The N6-threonylcarbamoyladenosine (t6A) modification at position 37 of ANN-decoding tRNAs is one of the few modifications that are found in the three domains of life. In the first half of the reaction, YrdC utilizes ATP, L-threonine and bicarbonate to synthesize an unstable intermediate TCA, whose threonylcarbamoyl-moiety is subsequently transferred onto the adenosine at position 37 of the substrate tRNAs by the cooperative action of three proteins YeaZ, YgjD and YjeE. In archaea and yeast, the transfer reaction requires the kinase, putative endopeptidase and other proteins of small size (KEOPS) protein complex, composed of Kae1, Bud32, Cgi121 and Pcc1, complemented by a fifth fungi-specific protein Gon7 in yeast. It is now well established that YgjD and its orthologs Kae1 and Qri7 are responsible for the catalysis of the transfer reaction. YgjD and YeaZ are forming a heterodimer that is capable of interacting with YjeE.

We report here the crystal structure of the heterodimer YgjD–YeaZ from E. coli in complex with ADP that is bound at the interfacial region of YeaZ. We cocrystallized the YgjD–YeaZ heterodimer with ATP and MgCl2 and determined the structure at a resolution of 2.3 Å. As expected we observed clear electron density for a nucleotide bound to two metal ions in the active site of YgjD, which we interpreted as Mg2+ and Fe2+/3+ based on electron density levels and X-ray fluorescence scanning at the Fe-edge (data not shown). The Mg2+ ion is located 6.2 Å away from the Fe2+/3+ ion and is liganded by the carboxylate side chains of Asp11 and Glu12, and close (3.7 Å) to the β-phosphate oxygen of the nucleotide. We did not observe electron density for the γ-phosphate group of ATP, which probably has been converted into ADP during the crystallization process. Interestingly, the Fo–Fc difference map calculated after structural refinement revealed an important residual electron density cloud situated at the YgjD–YeaZ interface. An ADP molecule could unequivocally fit the density and its refined B-factors were similar to those of the surrounding side chains. ADP is bound on top of the YeaZ helical bundle at the heterodimer interface. The β-phosphate is forming an ionic interaction with YeaZArg118 and the ribose 2′- and 3′-OH groups are forming hydrogen bonds with the YeaZHis34 side chain and the main chain carbonyl of YeaZArg32, both these residues are also very well conserved. The adenine base lies on top of a hydrophobic depression created at the interacting interface of YgjD–YeaZ (YeaZThr69 and YgjDLeu89) but does not form any specific H-bond interactions with the heterodimer.

>[2x]MRVLGIETSCDETGIAIYDDEKGLLANQLYSQVKLHADYGGVVPELASRDHVRKTVPLIQAALKESGLTAKDIDAVAYTAGPGLVGALLVGATVGRSLAFAWDVPAIPVHHMEGHLLAPMLEDNPPEFPFVALLVSGGHTQLISVTGIGQYELLGESIDDAAGEAFDKTAKLLGLDYPGGPLLSKMAAQGTAGRFVFPRPMTDRPGLDFSFSGLKTFAANTIRDNGTDDQTRADIARAFEDAVVDTLMIKCKRALDQTGFKRLVMAGGVSANRTLRAKLAEMMKKRRGEVFYARPEFCTDNGAMIAYAGMVRFKAGATADLGVSVRPRWPLAELPAAHHHHHH;>MRILAIDTATEACSVALWNDGTVNAHFELCPREHTQRILPMVQDILTTSGTSLTDINALAYGRGPGSFTGVRIGIGIAQGLALGAELPMIGVSTLMTMAQGAWRKNGATRVLAAIDARMGEVYWAEYQRDENGIWHGEETEAVLKPEIVHERMQQLSGEWVTVGTGWQAWPDLGKESGLVLRDGEVLLPAAEDMLPIACQMFAEGKTVAVEHAEPVYLRNNVAWKKLPGKEHHHHHH[2x]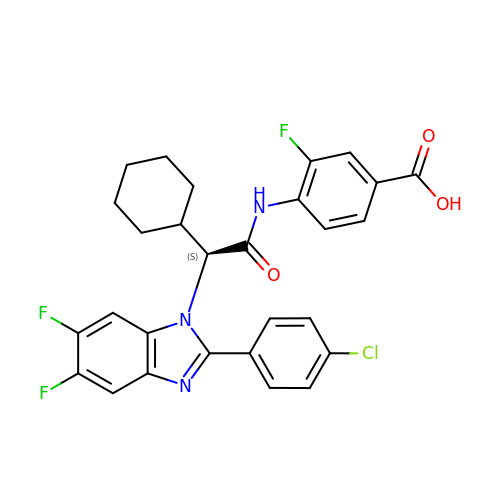4-({(2S)-2-[2-(4-chlorophenyl)-5,6-difluoro-1H-benzimidazol-1-yl]-2-cyclohexylacetyl}amino)-3-fluorobenzoic acid | C28 H23 Cl F3 N3 O3 | DGVNGMXASUNRAO-VWLOTQADSA-N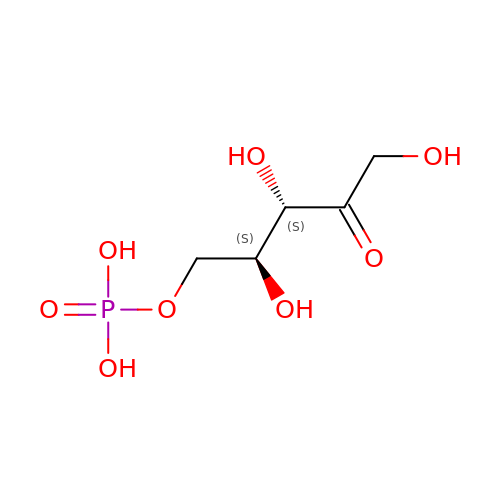5-O-phosphono-L-ribulose | C5 H11 O8 P | FNZLKVNUWIIPSJ-CRCLSJGQSA-N(1S,3R,5Z,7E,14beta,17alpha,20S)-20-[5-(1-hydroxy-1-methylethyl)furan-2-yl]-9,10-secopregna-5,7,10-triene-1,3-diol 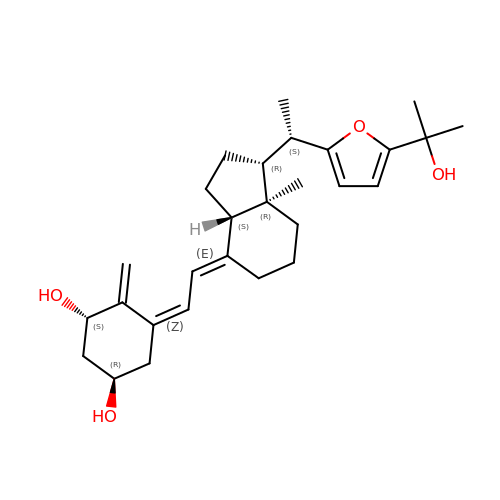| C28 H40 O4 | LQSIVELXOQAADQ-YQCVTLPCSA-N Human NAD-IDH is a key enzyme in the TCA cycle, which catalyzes the oxidative decarboxylation of ICT into α-KG. The α and β subunits form a heterodimer (αβ), and the α and γ subunits form another heterodimer (αγ), which are assembled into a heterotetramer (α2βγ) and further into a heterooctamer (the heterotetramer and heterooctamer are also called holoenzyme). Our previous biochemical studies demonstrated that the αγ heterodimer alone exhibits a high enzymatic activity and kinetic properties comparable with those of the holoenzyme and can be activated by CIT and ADP but inhibited by NADH; on the other hand, the αβ heterodimer alone exhibits a low activity and cannot be activated by the activators but can be inhibited by NADH. Our structural comparisons show that the αβ heterodimer has a similar yet more compact overall structure compared with the αγ heterodimer and contains a pseudo-allosteric site that exhibits substantial conformational differences from the allosteric site in the αγ heterodimer.

Crystals of the αβ heterodimer with the α subunit bound with an NAD at the active site (αNADβ) grew at condition II with the protein solution incubated with ICT and NAD (both 50 mm) before crystallization and belong to space group P21, and the structure was determined at 3.02 Å resolution with each asymmetric unit containing four αNADβ molecules, which form two dimers of heterodimers via the clasp domains. In this structure, there is clear electron density for an NAD but no electron density for Ca2+ or ICT at the active site. Like in the structures of NADP-IDHs, in the αNADβ structure, the cofactor NAD is bound at the deep pocket of the active site; the nicotinamide moiety is positioned in close to the ICT-binding site, and the adenine moiety is located at the far end of the active site. A number of strictly conserved residues from the large domain of the α subunit, including Lys-69A, Leu-72A, Thr-74A, and Asn-84A of the β3A-α3A loop and Glu-260A, Gly-264A, Thr-265A, Ala-266A, Asp-268A, and Asn-276A of the β12A-α8A loop, are involved in the binding of NAD via hydrogen-bonding interactions. In particular, the ribose 2′-OH of the adenosine moiety, which distinguishes NAD from NADP, is recognized by the side chain of Asp-268A via a hydrogen-bonding interaction, confirming the notion that Asp-268A of human NAD-IDH (or the equivalents of other NAD-IDHs) is the specificity determinant for NAD against NADP. Compared with the αCaβ structure, the NAD binding induces the conformational changes of the β3A-α3A loop and the β12A-α8A loop, yielding a closed active site. In addition, the side chain of Arg-88A on the β3A-α3A loop forms a hydrogen bond with the side chain of Tyr-126A on the β5A-β6A loop, which induces the side chain of Tyr-126A to assume the inactive conformation that is further stabilized by forming two hydrogen bonds with the side chains of Arg-119A and Asn-121A.

>GSTGGVQTVTLIPGDGIGPEISAAVMKIFDAAKAPIQWEERNVTAIQGPGGKWMIPSEAKESMDKNKMGLKGPLKTPIAAGHPSMNLLLRKTFDLYANVRPCVSIEGYKTPYTDVNIVTIRENTEGEYSGIEHVIVDGVVQSIKLITEGASKRIAEFAFEYARNNHRSNVTAVHKANIMRMSDGLFLQKCREVAESCKDIKFNEMYLDTVCLNMVQDPSQFDVLVMPNLYGDILSDLCAGLIGGLGVTPSGNIGANGVAIFESVHGTAPDIAGKDMANPTALLLSAVMMLRHMGLFDHAARIEAACFATIKDGKSLTKDLGGNAKCSDFTEEICRRVKDLD[4x];>[4x]ASRSQAEDVRVEGSFPVTMLPGDGVGPELMHAVKEVFKAAAVPVEFQEHHLSEVQNMASEEKLEQVLSSMKENKVAIIGKIHTPMEYKGELASYDMRLRRKLDLFANVVHVKSLPGYMTRHNNLDLVIIREQTEGEYSSLEHESARGVIECLKIVTRAKSQRIAKFAFDYATKKGRGKVTAVHKANIMKLGDGLFLQCCEEVAELYPKIKFETMIIDNCCMQLVQNPYQFDVLVMPNLYGNIIDNLAAGLVGGAGVVPGESYSAEYAVFETGARHPFAQAVGRNIANPTAMLLSASNMLRHLNLEYHSSMIADAVKKVIKVGKVRTSDMGGYATCHDFTEEICRRVKDLDENLYFQ>[2x]SNASDESDLPSAMPAVPAFGVEERNMVSGVLTLAERSIRSIMTPRTDVSWVNIDDDAATIRQQLTAAPHSFFPVCRGSLDEVVGIGRAKDLVA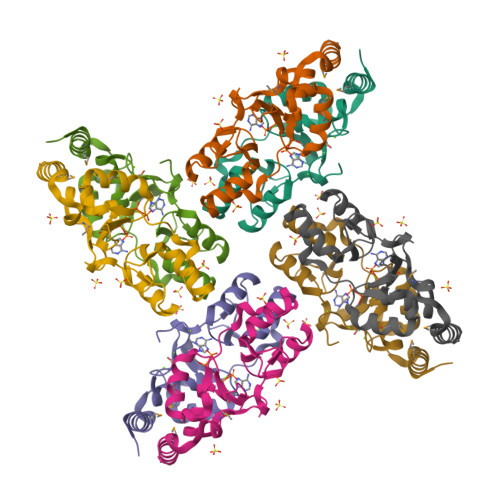DLITEGRVRRNRLRDPIIVHESIGILRLMDTLKRSRGQLVLVADEFGAIEGLVTPIDVFEAIAGEFPDEDELPDIVAESE> HPETLVKVKDAEDQLGARVGYIELDLNSGKILESFRPEERFPMMSTFKVLLCGAVLSRVDAGQEQLGRRIHYSQNDLVEYSPVTEKHLTDGMTVRELCSAAITMSDNTAANLLLTTIGGPKELTAFLHNMGDHVTRLDRWEPELNEAIPNDERDTTMPAA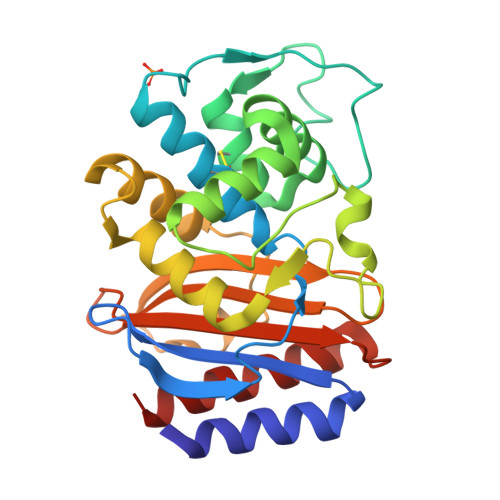MATTLRKLLTGELLTPASRQQLIDWMEADKVAGPLLRSALPAGWFIADKSGAGERGSRGIIAALGPDGKPSRIVVIYTTGSQATMDERNRQIAEIGASLIKHW> GCGAA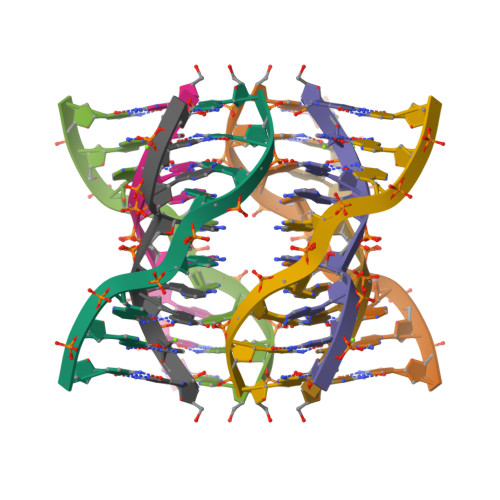AGC>[2x]KIRPECFELLRVLGKGGYGKVFQVRKVTGANTGKIFAMKVLKKAMIVRNAKDTAHTKAERNILEEVKHPFIVDLIYAFQTGGKLYLILEYLSGGELFMQLEREGIFMEDTACFYLAEISMALGHLHQKGIIYRDLKPENIMLNHQGHVKLTDFGLCKESIH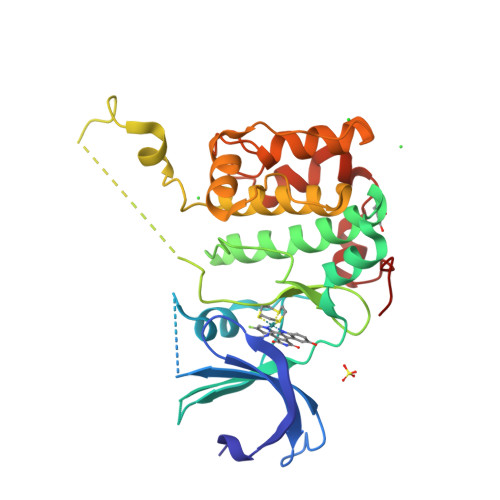DGTVTHTFCGTIEYMAPEILMRSGHNRAVDWWSLGALMYDMLTGAPPFTGENRKKTIDKILKCKLNLPPYLTQEARDLLKKLLKRNAASRLGAGPGDAGEVQAHPFFRHINWEELLARKVEPPFKPL Bromodomains (BRDs) are protein interaction modules that specifically recognize ε-N-lysine acetylation motifs, a key event in the reading process of epigenetic marks. The 61 BRDs in the human genome cluster into eight families based on structure/sequence similarity. Despite large sequence variations, all BRD modules share a conserved fold that comprises a left-handed bundle of four α helices (αZ, αA, αB, αC), linked by loop regions of variable length (ZA and BC loops), which line the Kac binding site and determine binding specificity. The four helices form a deep cavity that is extended by the two loop regions (ZA and BC loops), creating a largely hydrophobic Kac binding pocket.

BRDs are evolutionarily conserved and present in diverse nuclear proteins comprising HATs (GCN5, PCAF), ATP-dependent chromatin-remodeling complexes (BAZ1B), helicases (SMARCA), methyltransferases (MLL, ASH1L), transcriptional coactivators (TRIM/TIF1, TAFs) transcriptional mediators (TAF1), nuclear-scaffolding proteins (PB1), and the BET family (Muller et al., 2011). The nuclear body protein SP140 as well as the related protein LOC93349 and PCAF showed nonspecific binding to most peptides.

>[2x]SMGKEKSKEPRDPDQLYSTLKSILQQVKSHQSAWPFMEPVKRTEAPGYYEVIRFPMDLKTMSERLKNRYYVSKKLFMADLQRVFTNCKEYNPPESEYYKCANILEKFFFSKIKEAGLID>[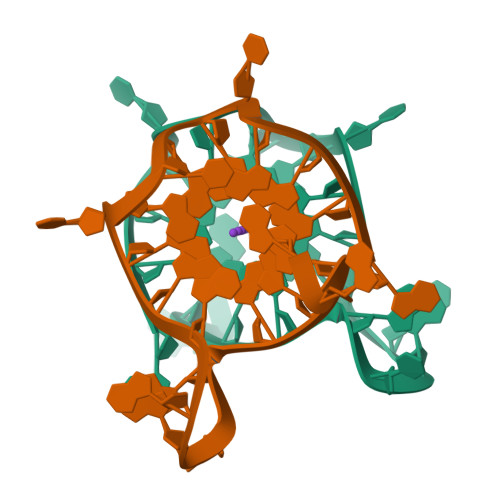2x]AGGGCGGTGTGGGAATAGGGAA>[6x]XGEIAQGLKEIA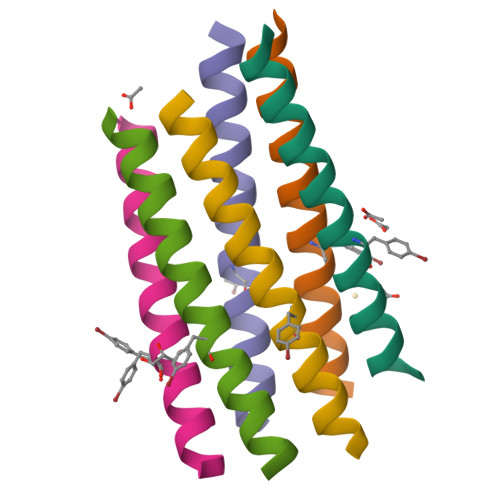KGLKEIAYGLKEIAQGLKGX> TNTPEQDRYLQAKKYIEFYVVVDNIMYRHYKRDQPVIKRKVYEMINTMNMIYRRLNFHIALIGLEIWSNINEINVQSDVRATLNLFGEWREKKLLPRKRNDNAQLLTGIDFNGTPVGLAYIGSICNPKTSAAVVQDYSSRTRMVAITMAHEMGHNLGMNHDRGFCTCGFNKCVMSTRRTKPAYQFSSCSVREHQRYLLRDRPQCILNKPLSTDIVSPPICGNYFVEVGEECDCGSPADCQSACCNATTCKLQHEAQCDSEECCEKCKFKGARAECRAA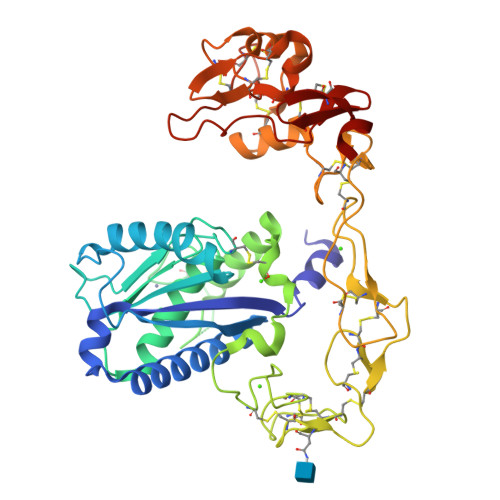KDDCDLPELCTGQSAECPTDVFQRNGLPCQNNQGYCYNGKCPIMTNQCIALRGPGVKVSRDSCFTLNQRTRGCGLCRMEYGRKIPCAAKDVKCGRLFCKRRNSMICNCSISPRDPNYGMVEPGTKCGDGMVCSNRQCVDVKTAY>[6x]MFKMKVEDYFHDILRERKIHLTLIDPEEQTPEEAVEIARAAIRGGTDGIMLGGSTTDSSELDNTARALRENIDVPIILFPGNTTGVSRYADAIFFMSLLNSTNPYWEIGAQALGAA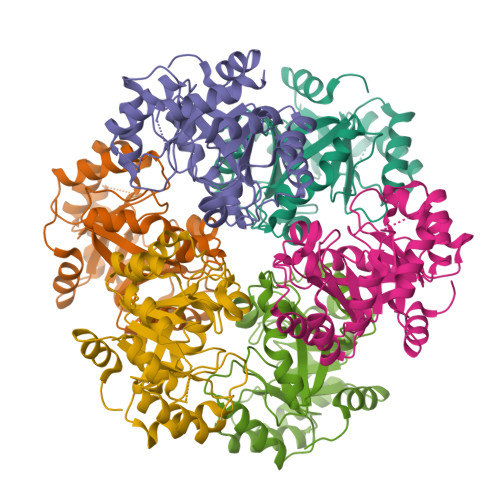TVKKMGIEALPMGYLVVEPGGTVGWVGDTKPVPRNKPDIAAAYAMAAEFLGMRLFYLEAGSGAPEHVPEEMIALVKRCTDQILIVGGGIRSGEDAARVAGAGADVVVTGTVVENSDNVEDKIREIVEGMGSVLEHHHHHH>[2x]MGSDKIHHHHHHMKVQYECLTCMANQCQRIVEMATQDMDIRRRAMILAAKLLAKEYNENAIPAIAGSLIFLELYKFLGNDDPFIEYKLKSEEMARKVADIIKRKLKLDFELAVKLAIIGNVIDFSVGFSPEDLEEEVEKMLKDKLYIDDSKELFEEVKRAENILYIT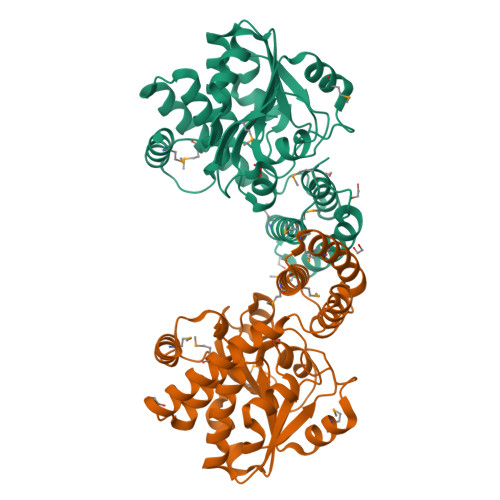DNVGEHYFDAILIEKIREISNAEVYIAGKEGPIINDATVEDLKRAGLEKLGKVISTGTRIVGVPLKLVSREFMEAFNKADVIIAKGQGNFETLSEINDSRIFFLLKAKCPAVARELKVPKGALVCMRNKFKL> TMAASQTSQTVASHVPFADLCSTLERIQKSKGRAEKIRHFREFLDSWRKFHDALHKNHKDVTDSFYPAMRLILPQLERERMAYGIKETMLAKLYIELLNLPRDGKDALKLLNYRTPTGTHGDAGDFAMIAYFVLKPRCLQKGSLTIQQVNDLLDSIASNNSAKRKDLIKKSLLQLITQSSALEQKWLIRMIIKDLKLGVSQQTIFSVFHNDAAELHNVTTDLEKVCRQLHDPSVGLSDISITLFSAFKPMLAAIADIEHIEKDMKHQSFYIETKLDGERMQMHKDGDVYKYFSRNGYNYTDQFGASPTEGSLTPFIHNAFKADIQICILDGEMMAYNPNTQTFMQKGTKFDIKRMVEDSDLQTCYCVFDVLMVNNKKLGHETLRKRYEILSSIFTPIPGRIEIVQKTQAHTKNEVIDALNEAIDKREEGIMVKQPLSIYKPDKRGEGWLKIKPEYVSGLMDELDILIVGGYWGKGSRGGMMSHFLCAVAEKPPPGEKPSVFHTLSRVGSGCTMKELYDLGLKLAKYWKPFH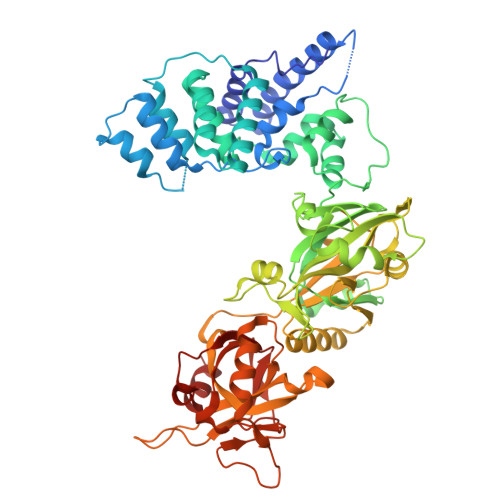RKAPPSSILCGTEKPEVYIEPCNSVIVQIKAAEIVPSDMYKTGCTLRFPRIEKIRDDKEWHECMTLDDLEQLRGKASGK(2R,4R,5R)-2,4,5-trimethyl-1,3-oxazolidine | C6 H13 N O | 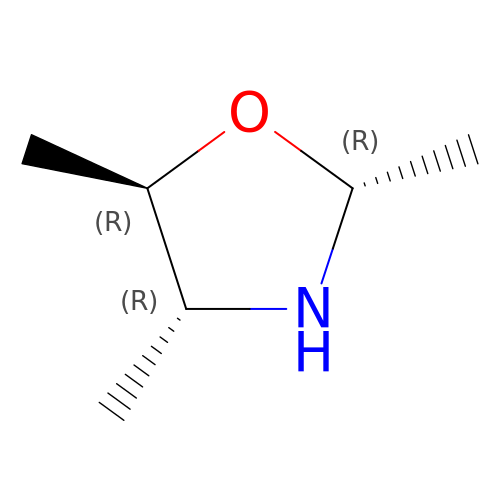KGOJHIRKYWXNFA-HSUXUTPPSA-N Cell division in most bacteria is regulated by the tubulin homolog FtsZ as well as ZapA, a FtsZ-associated protein. In the presence of GTP, FtsZ polymerizes into protofilaments, which further associate into a ring-like structure (the Z-ring). ZapA binds FtsZ straight protofilaments preferentially to crosslink FtsZ protofilaments; thereby, ZapA bundles more aligned and straight filaments constituting a coherent Z-ring. A FtsZ protofilament has polarity and lacks symmetry, while ZapA is in an equilibrium between homodimer and homotetramer, which are related by C2 and D2 symmetry, respectively.

To acquire the structural information of the missing dimer head, we determined the crystal structure of K. pneumoniae ZapA (KpZapA) at 1.8 Å resolution and performed a structural comparison of ZapA within the ZapA-FtsZ complex with the crystal structures of KpZapA, E. coli ZapA (EcZapA, PDB code: 4P1M18), and P. aeruginosa ZapA (PaZapA, PDB code: 1W2E10). The cryo-EM structure of KpZapA within the ZapA-FtsZ complex was superimposed well to the crystal structures of KpZapA and EcZapA (r.m.s.d. = 0.851 Å among 128 Cα atom for KpZapA, and 0.911 Å among 127 Cα atom for EcZapA). For the dimer head on the missing side, KpZapA and EcZapA overlapped well, but PaZapA did not. The N-terminal tail of FtsZ in our cryo-EM structure, which is sandwiched by two ZapA molecules, overlaps with the C-terminal tail of KpZapA and EcZapA. This observation indicates that the C-terminal tail of ZapA moves aside to accept the N-terminal tail of FtsZ when the ZapA-FtsZ complex forms. Furthermore, the α1-α2 loop of ZapA undergoes a conformational change to recognize the N-terminal tail of FtsZ.

>[2x]MSAQPVDLQIFGRSLRVNCPPEQRDALNQAAEDLNQRLQDLKERTRVTNTEQLVFIAALNISYELTQEKAKTRDYASSMEQRIRMLQQTIEQALLEQGRISERPGSKFE> MVSTTQSRSLKAMGEEIWKNKTEKINTELFTLTYGSIVAQLCQDYERDFNKVNDHLYSMGYNIGCRLIEDFLARTALPRCENLVKTSEVLSKCAFKIFLNITPNITNWSHN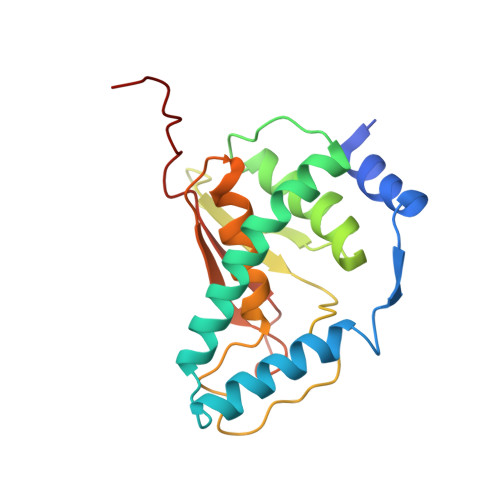KDTFSLILDENPLADFVELPMDAMKSLWYSNILCGVLKGSLEMVQLDCDVWFVSDILRGDSQTEIKVKLNRILKDEIPIG PAPP-A and its paralog PAPP-A2 are metalloproteases that mediate IGF bioavailability through cleavage of IGF binding proteins (IGFBPs). Secreted PAPP-A is a 1547-residue, multidomain, dimeric glycoprotein which recognizes and cleaves IGFBP2, 4 and 510–17, while PAPP-A2 mainly cleaves IGFBP3 and 59,17–21. The proteolytic cleavage of IGFBPs is required for the release of sequestered IGFs to enable their binding to insulin-like growth factor receptors (IGFRs) for downstream signaling. We show that PAPP-A is a flexible trans-dimer that binds IGFBP5 via a 25-amino acid anchor peptide which extends into the metalloprotease active site.

To facilitate the understanding of IGFBP5 recognition, we further obtained the cryo-EM map of substrate-unbound PAPP-A (E483A) at ~3.35 Å. This substrate-unbound map exhibits dimer configuration, but with a much lower resolution for the second monomer (chain A) compared with PAPP-ABP5, and multi-body refinement suggested this should be due to the even larger movement between the two monomers. Nevertheless, we were able to reconstitute the complete structure for one monomer and a partial structure for the second monomer. Same as the PAPP-ABP5, the substrate-unbound PAPP-A structure shows the trans-dimer configuration. To examine whether substrate binding introduces conformational changes to PAPP-A, we overlaid the structure of the substrate-unbound PAPP-A with the structure of PAPP-ABP5. The two structures share the same overall domain architecture and no obvious conformational change was observed in the IGFBP5 binding groove. There were slight differences in some loops around the substrate binding groove, but this is likely due to the limited resolution and the flexibility of these loops rather than representing specific conformational differences. However, there may be subtle differences in substrate binding due to this mutation that we are not able to distinguish. As aforementioned, multibody refinement of PAPP-ABP5 and substrate-unbound PAPP-A showed that in the later structure, the two monomers have more obvious rotation, suggesting the substrate association helps to stabilize the PAPP-A trans-dimer. While we used the catalytically inactive PAPP-A (E483A) for structure work, the Zn2+ coordination remains intact, which is a validation of the state of the active site.

>[2x]REARGATEEPSPPSRALYFSGRGEQLRLRADLELPRDAFTLQVWLRAEGGQRSPAVITGLYDKCSYISRDRGWVVGIHTISDQDNKDPRYFFSLKTDRARQVTTINAHRSYLPGQWVYLAATYDGQFMKLYVNGAQVATSGEQVGGIFSPLTQKCKVLMLGGSALNHNYRGYIEHFSLWKVARTQREILSDMETHGAHTALPQLLLQENWDNVKHAWSPMKDGSSPKVEFSNAHGFLLDTSLEPPLCGQTLCDNTEVIASYNQLSSFRQPKVVRYRVVNLYEDDHKNPTVTREQVDFQHHQLAEAFKQYNISWELDVLEVSNSSLRRRLILANCDISKIGDENCDPECNHTLTGHDGGDCRHLRHPAFVKKQHNGVCDMDCNYERFNFDGGECCDPEITNVTQTCFDPDSPHRAYLDVNELKNILKLDGSTHLNIFFAKSSEEELAGVATWPWDKEALMHLGGIVLNPSFYGMPGHTHTMIHAIGHSLGLYHVFRGISEIQSCSDPCMETEPSFETGDLCNDTNPAPKHKSCGDPGPGNDTCGFHSFFNTPYNNFMSYADDDCTDSFTPNQVARMHCYLDLVYQGWQPSRKPAPVALAPQVLGHTTDSVTLEWFPPIDGHFFERELGSACHLCLEGRILVQYASNASSPMPCSPSGHWSPREAEGHPDVEQPCKSSVRTWSPNSAVNPHTVPPACPEPQGCYLELEFLYPLVPESLTIWVTFVSTDWDSSGAVNDIKLLAVSGKNISLGPQNVFCDVPLTIRLWDVGEEVYGIQIYTLDEHLEIDAAMLTSTADTPLCLQCKPLKYKVVRDPPLQMDVASILHLNRKFVDMDLNLGSVYQYWVITISGTEESEPSPAVTYIHGSGYCGDGIIQKDQGEQCDDMNKINGDGCSLFCRQEVSFNCIDEPSRCYFHDGDGVCEEFEQKTSIKDCGVYTPQGFLDQWASNASVSHQDQQCPGWVIIGQPAASQVCRTKVIDLSEGISQHAWYPCTISYPYSQLAQTTFWLRAYFSQPMVAAAVIVHLVTDGTYYGDQKQETISVQLLDTKDQSHDLGLHVLSCRNNPLIIPVVHDLSQPFYHSQAVRVSFSSPLVAISGVALRSFDNFDPVTLSSCQRGETYSPAEQSCVHFACEKTDCPELAVENAYLNCSSSDRYHGAQCTVSCRTGYVLQIRRDDELIKSQTGPSVTVTCTEGKWNKQVACEPVDCSIPDHHQVYAASFSCPEGTTFGSQCSFQCRHPAQLKGNNSLLTCMEDGLWSFPEALCELMCLAPPPVPNADLQTARCRENKHKVGSFCKYKCKPGYHVPGSSRKSKKRAFKTQCTQDGSWQEGACVPVTCDPPPPKFHGLYQCTNGFQFNSECRIKCEDSDASQGLGSNVIHCRKDGTWNGSFHVCQEMQGQCSVPNELNSNLKLQCPDGYAIGSECATSCLDHNSESIILPMNVTVRDIPHWLNPTRVERVVCTAGLKWYPHPALIHCVKGCEPFMGDNYCDAINNRAFCNYDGGDCCTSTVKTKKVTPFPMSCDLQGDCACRDPQAQEHSRKDLRGYSHGSGPTRTRPLEQKLISEEDLAANDILDYKDDDDKV> EDKQERANYEKLQQKFQMLMSKHQAHVRPQFESLEKINKDIVGWIKLSGTSLNYPVLQGKTNHDYLNLDFEREHRRKGSIFMDFRNELKNLNHNTILYGHHVGDNTMFDVLEDYL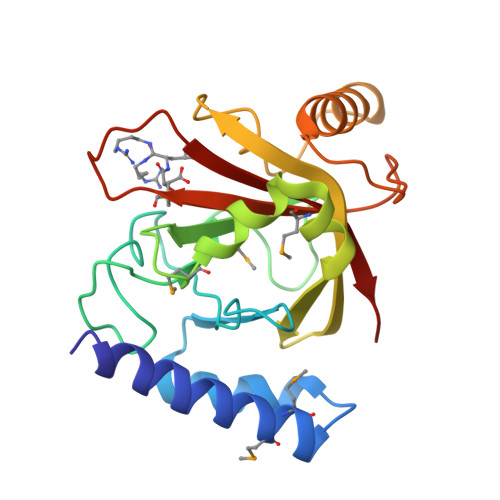KQSFYEKHKIIEFDNKYGKYQLQVFSAYKTTTKDNYIRTDFENDQDYQQFLDETKRKSVINSDVNVTVKDRIMTLSTCEDAYSETTKRIVVVAKIIKVS> GSPGTPEVKVASSEDVDLPCTAPWDPQVPYTVSWVKLLEGGEERMETPQEDHLRGQHYHQKGQNGSF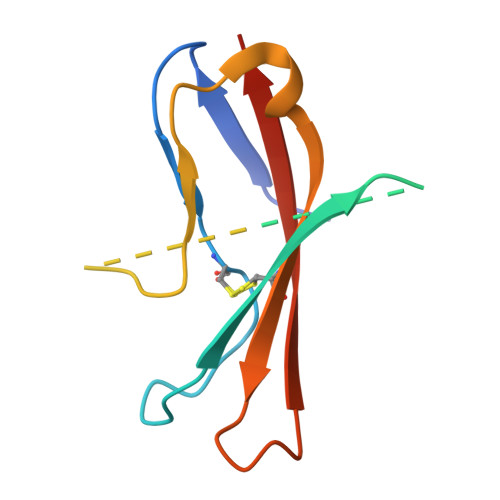DAPNERPYSLKIRNTTSSNSGTYRCTLQDPDGQRNLSGKVILRVTGSPA>KSPSAQELKEQGNRLFVGRKYPEAAACYGRAITRNPLVAVYYTNRALCYLKMQQHEQALADCRRALELDGQSVKAHFFLGQCQLEMESYDEAIANLQRAYSLAKEQRLNFGDDIPSALRIAKKKRWNS[2x];>[2x]SSTGSIDMVD

Many studies have suggested that CHIP (C-terminus of Hsc70 interacting protein; STUB1) is one of the major E3 ubiquitin ligases responsible for degradation of tau5. TauC3 is the product of caspase cleavage at aspartate 421 (D421) in tau and multiple lines of evidence suggest that this truncation plays an important role in neurodegenerative disease. To explore these questions, we focus on a cleaved proteoform of tau (tauC3), which selectively accumulates in AD and was recently shown to be degraded by its direct binding to the E3 ubiquitin ligase, CHIP. Here, we find that phosphorylation of tauC3 at a single residue, pS416, is sufficient to weaken its interaction with CHIP.

A 1.8 Å crystal structure of the CHIP TPR domain bound to a 10-mer tauC3 C-terminal peptide. Key molecular contacts with side chains were also maintained, such as the “carboxylate clamp” interactions, involving coordination of tauC3’s Asp421 side chain and carboxylate-terminus by cationic Lys30 and Lys95 side chains in CHIP’s TPR domain. However, we did note a few distinct interactions, including between tauC3’s Asp418 and CHIP’s Lys72. Critically, this co-structure also suggested why phosphorylation of S416 weakens binding to CHIP. Specifically, we noted that tauC3’s Ser416 was in close proximity with CHIP’s Asp134. Thus, phosphorylation of tauC3’s S416 would be expected to create interference at this site, likely involving both steric and electrostatic clashes. To test this idea, we mutated CHIP’s Asp134 (D134A) or the adjacent Phe131 residue (F131A), to alanine and tested binding of these CHIP variants to tauC3 peptides. Fortunately, installing D134A into CHIP was tolerated; for example, it bound normally to WT tauC3 in DSF experiments. To independently verify this finding, we performed FP assays and confirmed that CHIP D134A bound normally to WT tauC3 (Ki 5.57 ± 0.34 µM) and that it regained the ability to bind phosphorylated tauC3 peptide (Ki 1.84 ± 0.23 µM). Together, these results support a model in which phosphorylation at S416 weakens binding to CHIP via clashes with D134 in the TPR domain.>MAHHHHHHSSGLEVLFQGPMNESVKEIPDVLKSQCGFNCLTDISHSSFNEFRQQVSEHLSWSETHDLYHDAQQAQKDNRLYEARILKRANPQLQNAVHLAILAPNAELIGYNNQFSGRASQYVAPGTVSSMFSPAAYLTELYREARNLHASDSVYYLDTRRPDLKSMALSQQNMDIELSTLSLSNELLLESIKTESKLENYTKVMEMLSTFRPSGATPYHDAYENVREVIQLQDPGLEQLNASPAIAGLMHQASLLGINASISPELFNILTEEITEGNAEELYKKNFGNIEPASLAMPEYLKRYYNLSDEELSQFIGKASNFGQQE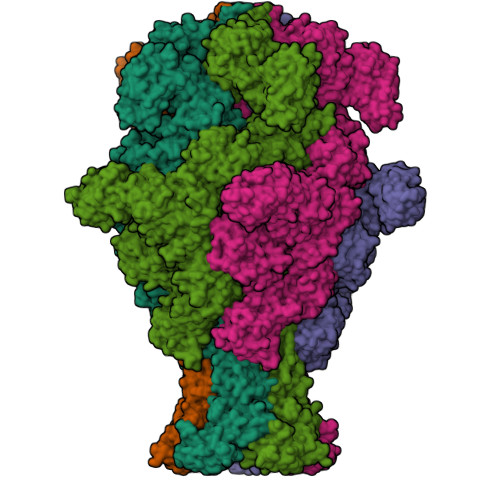YSNNQLITPVVNSSDGTVKVYRITREYTTNAYQMDVELFPFGGENYRLDYKFKNFYNASYLSIKLNDKRELVRTEGAPQVNIEYSANITLNTADISQPFEIGLTRVLPSGSWAYAAAKFTVEEYNQYSFLLKLNKAIRLSRATELSPTILEGIVRSVNLQLDINTDVLGKVFLTKYYMQRYAIHAETALILCNAPISQRSYDNQPSQFDRLFNTPLLNGQYFSTGDEEIDLNSGSTGDWRKTILKRAFNIDDVSLFRLLKITDHDNKDGKIKNNLKNLSNLYIGKLLADIHQLTIDELDLLLIAVGEGKTNLSAISDKQLATLIRKLNTITSWLHTQKWSVFQLFIMTSTSYNKTLTPEIKNLLDTVYHGLQGFDKDKADLLHVMAPYIAATLQLSSENVAHSVLLWADKLQPGDGAMTAEKFWDWLNTKYTPGSSEAVETQEHIVQYCQALAQLEMVYHSTGINENAFRLFVTKPEMFGAATGAAPAHDALSLIMLTRFADWVNALGEKASSVLAAFEANSLTAEQLADAMNLDANLLLQASIQAQNHQHLPPVTPENAFSCWTSINTILQWVNVAQQLNVAPQGVSALVGLDYIQSMKETPTYAQWENAAGVLTAGLNSQQANTLHAFLDESRSAALSTYYIRQVAKAAAAIKSRDDLYQYLLIDNQVSAAIKTTRIAEAIASIQLYVNRALENVEENANSGVISRQFFIDWDKYNKRYSTWAGVSQLVYYPENYIDPTMRIGQTKMMDALLQSVSQSQLNADTVEDAFMSYLTSFEQVANLKVISAYHDNINNDQGLTYFIGLSETDAGEYYWRSVDHSKFNDGKFAANAWSEWHKIDCPINPYKSTIRPVIYKSRLYLLWLEQKEITWQTGNSKDGYQTETDYRYELKLAHIRYDGTWNTPITFDVNKKISELKLEKNRAPGLYCAGYQGEDTLLVMFYNQQDTLDSYKNASMQGLYIFADMASKDMTPEQSNVYRDNSYQQFDTNNVRRVNNRYAEDYEIPSSVSSRKDYGWGDYYLSMVYNGDIPTINYKAASSDLKIYISPKLRIIHNGYEGQKRNQCNLMNKYGKLGDKFIVYTSLGVNPNNSSNKLMFYPVYQYSGNTSGLNQGRLLFHRDTTYPSKVEAWIPGAKRSLTNQNAAIGDDYATDSLNKPDDLKQYIFMTDSKGTATDVSGPVEINTAISPAKVQIIVKAGGKEQTFTADKDVSIQPSPSFDEMNYQFNALEIDGSGLNFINNSASIDVTFTAFAEDGRKLGYESFSIPVTLKVSTDNALTLHHNENGAQYMQWQSYRTRLNTLFARQLVARATTGIDTILSMETQNIQEPQLGKGFYATFVIPPYNLSTHGDERWFKLYIKHVVDNNSHIIYSGQLTDTNINITLFIPLDDVPLNQDYHAKVYMTFKKSPSDGTWWGPHFVRDDKGIVTINPKSILTHFESVNVLNNISSEPMDFSGANSLYFWELFYYTPMLVAQRLLHEQNFDEANRWLKYVWSPSGYIVHGQIQNYQWNVRPLLEDTSWNSDPLDSVDPDAVAQHDPMHYKVSTFMRTLDLLIARGDHAYRQLERDTLNEAKMWYMQALHLLGDKPYLPLSTTWSDPRLDRAADITTQNAHDSAIVALRQNIPTPAPLSLRSANTLTDLFLPQINEVMMNYWQTLAQRVYNLRHNLSIDGQPLYLPIYATPADPKALLSAAVATSQGGGKLPESFMSLWRFPHMLENARGMVSQLTQFGSTLQNIIERQDAEALNALLQNQAAELILTNLSIQDKTIEELDAEKTVLEKSKAGAQSRFDSYGKLYDENINAGENQAMTLRASAAGLTTAVQASRLAGAAADLVPNIFGFAGGGSRWGAIAEATGYVMEFSANVMNTEADKISQSETYRRRRQEWEIQRNNAEAELKQIDAQLKSLAVRREAAVLQKTSLKTQQEQTQSQLAFLQRKFSNQALYNWLRGRLAAIYFQFYDLAVARCLMAEQAYRWELNDDSARFIKPGAWQGTYAGLLAGETLMLSLAQMEDAHLKRDKRALEVERTVSLAEVYAGLPKDNGPFSLAQEIDKLVSQGSGSAGSGNNNLAFGAGTDTKTSLQASVSFADLKIREDYPASLGKIRRIKQISVTLPALLGPYQDVQAILSYGDKAGLANGCEALAVSHGMNDSGQFQLDFNDGKFLPFEGIAIDQGTLTLSFPNASMPEKGKQATMLKTLNDIILHIRYTIK[5x]N-benzyl-3-(2-cyano-6-propylpyrimidin-4-yl)-N-[2-(dimethylamino)ethyl]-5-(trifluoromethyl)benzamide 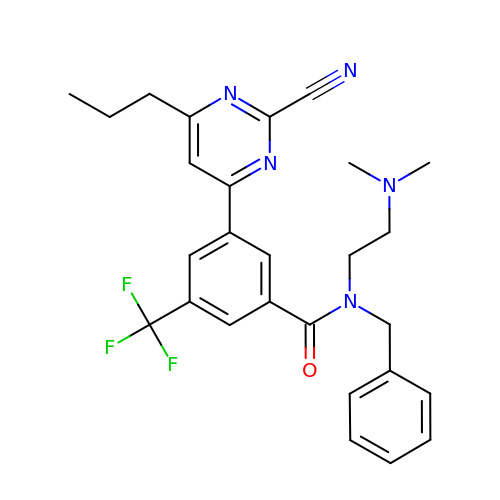| C27 H28 F3 N5 O | AGGVJWZHDDIPAU-UHFFFAOYSA-N> SNSLHWPTSLPSGDAFSSVGTHRFVQKVEEMVQNHMTYSLQDVGGDANWQLVVEEGEMKVYRREVEENGIVLDPLKATHAVKGVTGHEVCNYFWNVDVRNDWETTIENFHVVETLADNAIIIYQTHKRVWPASQRDVLYLSVIRKIPALTENDPETWIVCNFSVDHDSAPLNNRCVRAKINVAMICQTLVSPP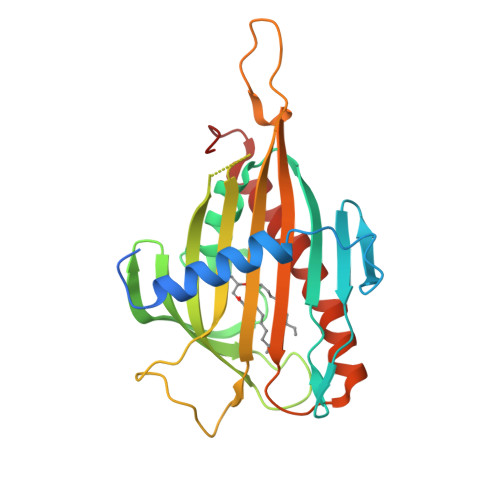EGNQEISRDNILCKITYVANVNPGGWAPASVLRAVAKREYPKFLKRFTSYVQEKTAGKPILF> 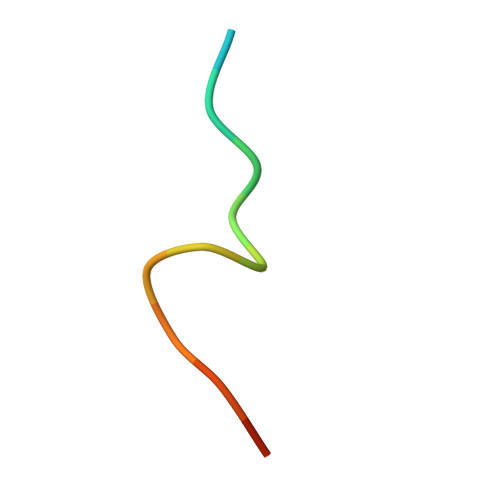MEQRRVTDFFARRR> TGYVSTMPKVIIFTDFDGTVTGKSGNETVFTEFYQSLLQGYKKDVEQDYKNTPMKDPIEAQALFEAKYGKYNENFDHDQQDVDFLMSPEAVAFFHEVLKNDDVTVNIVTKNRAEYIKAVFKYQGFSDEEISKLTILES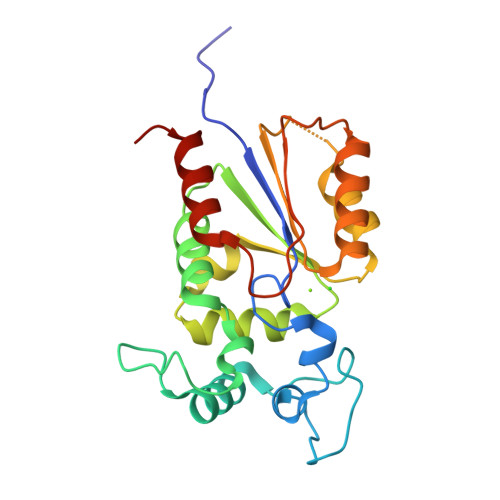GYKFNDVNSRLNHPTERANRVYILDDSPTDYAEMLRAVKGKGYNEEEIRGYRKNPGEFEWSQYLEDVREMFPPKEN> DMRPEIWI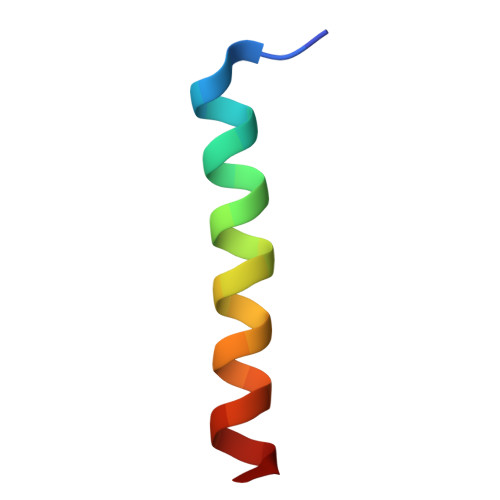AQELRRXGDEFNAYYARR>[2x]SEFELGAPATRSAGQQATVDRLRTQVTGFLSGALGKLQALSAQNMDPELAQFRVLDVDRAIMPLLIVAENARNP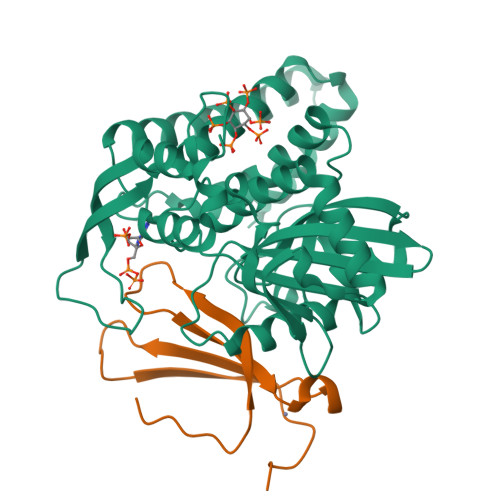GLNLVPLHMDMAEDEEVRTQPPMAGSRHIAEFVASARPGRYRAVIDDGSHTRAADIRKDASGTSVIVVDPLRKEKDESAYVDYADNVNMEFGEHAKCAFIPVDIQKSFFDCRILSLSLALKMHDKDDAFAAFHETLRNGGDPSHHVSRAQQTEELGATLVLDGAPLVDARMMKHGQAASSVSRYLGNHPEQSTVPVNKRNETLGERTTRHLVKRKVRNRADSEGRVTSGETKEITFSNSVEQKRIALLNRAASYVNSAPPPVVMRMAKLLQDSLLDTN;>[2x]SESKVKKVVSIPAIDEGDLWTWRKYGQKDILGSRFPRGYYRCAYKFTHGCKATKQVQRSETDSNMLAITYLSEHNHPRPT> GPLGSKSLVDTVYALKDEVQELR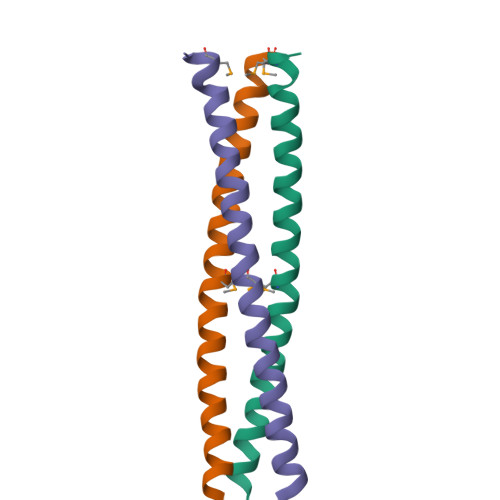QDNKKMKKSLEEEQRARKDLEKLVRKVLKNMND> ASVHGTTYELLRRQGIDTVFGNPGSNELPFLKDFPEDFRYILALQEACVVGIADGYAQASRKPAFINLASAAGTGNAMGALSNAWNSHSPLIVTAGQQTRAMIGVEALLTNVDAANLPRPLVKWSYEPASAAEV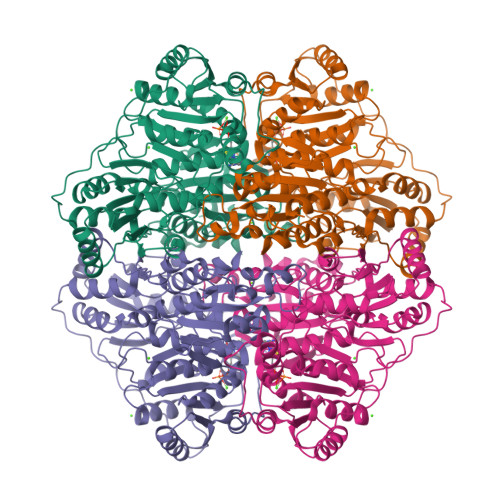PHAMSRAIHMASMAPQGPVYLSVPYDDWDKDADPQSHHLFDRHVSSSVRLNDQDLDILVKALNSASNPAIVLGPDVDAANANADCVMLAERLKAPVWVAPSAPRCPFPTRHPCFRGLMPAGIAAISQLLEGHDVVLVIGAPVFRYHQYDPGQYLKPGTRLISVTCDPLEAARAPMGDAIVADIGAMASALANLVEESSRQLPTAAPEPAKVDQDAGRLHPETVFDTLNDMAPENAIYLNESTSTTAQMWQRLNMRNPGSYYFCAAGGLGFALPAAIGVQLAEPERQVIAVIGDGSANYSISALWTAAQYNIPTIFVIMNNGTYGALRWFAGVLEAENVPGLDVPGIDFRALAKGYGVQALKADNLEQLKGSLQEALSAKGPVLIEVSTVS> GEKRKSRQAEVNIGMVGHVDHGKTTLTKALTGVWTDTHSEELRRGITIKIGFADAEIRRCPNCGRYSTSPVCPYCGHETEFVRRVSFIDAPGHEALMTTMLAGASLMDGAILVIAANEPCPRPQTREHLMALQIIGQK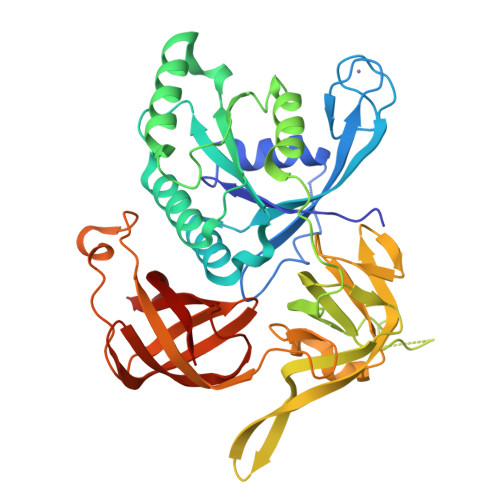NIIIAQNKIELVDKEKALENYRQIKEFIEGTVAENAPIIPISALHGANIDVLVKAIEDFIPTPKRDPNKPPKMLVLRSFDVNKPGTPPEKLVGGVLDGSIVQGKLKVGDEIEIRPGVPYEEHGRIKYEPITTEIVSLQAGGQFVEEAYPGGLVGVGTKLDPYLTKGDLMAGNVVGKPGKLPPVWDSLRLEVHLLERVVGTEQELKVEPIKRKEVLLLNVGTARTMGLVTGLGKDEIEVKLQIPVCAEPGDRVAISRQIGSRWRLIGYGIIKE> MGVEKVPKYDIPTKKVDYVFIELDKMKPHQQLVQKELEAFIESVTGSGIFWKPMLLAKVPGEDMYLIVDGHHRWAGLQKLGAKRAPSVILDYFSDDVKVYTWYPAFKGDLNEVVERLKKEGLEVIEDPEAEEKAERGEIAFALVGEKSFAIPGGLEEQKKVSKVLDEMSVEGKIELIYYG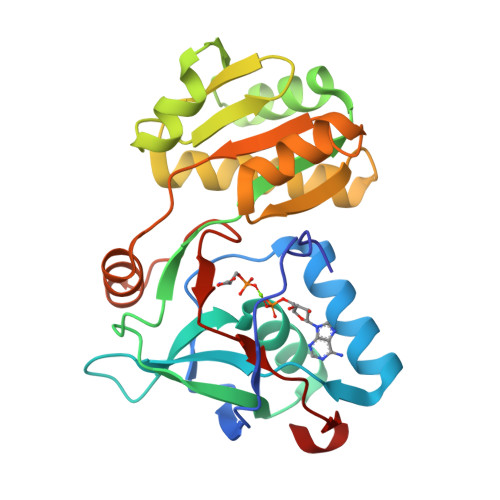LKEDAREDMAKGEIDYVFIRKAPTKEEVMELVKRGEVYSPKTTRHVLPFNPDKIDVKLEELF> GYGR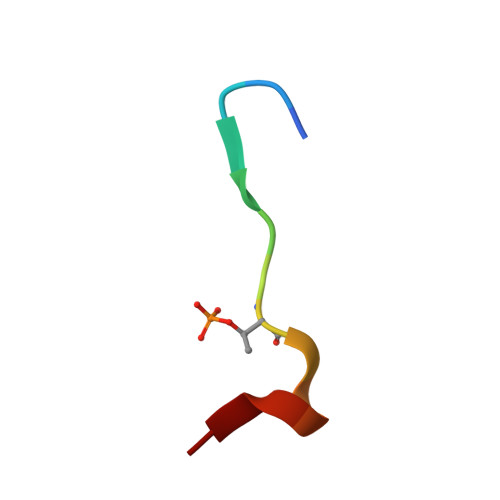VESTPPAFLP> GPLSLSVDAFKILEDPKWEFPRKNLVLGKTLGEGEFGKVVKATAFHLKGRAGYTTVAVKMLKENASPSELRDLLSEFNVLKQVNHPHVIKLYGACSQDGPLLLIVEYAKYGSLRGFLRESRKVGPGYPDERALTMGDLISFAWQISQGMQYLAEMKLVHRDLAARNILVAEGRKMKISDFGLSRDVYEEDSYVKRSQGRIPVKWMAIESLFDHIYTTQSDVWSFGVLLWEIVTLGGNPYPGIPPERLFNLLKTGHRMERPDNCSEEMYRLMLQCWKQEPDKRPVFADISKDLEKMMVKR

RET (REarranged during Transfection) is a receptor tyrosine kinase (RTK) that is required for normal development, maturation and maintenance of several tissues and cell types. Gain of function mutations in RET are implicated in several human cancers, e.g. medullary thyroid cancer (MTC) and lung adenocarcinoma (LAD). The identification of these mutations and rearrangements in RET which lead to constitutive activation, together with convincing preclinical data validating RET as a classical oncogene, make this kinase an attractive target for cancer therapy. Our initial focus was to identify novel, low molecular weight, ATP-competitive inhibitors of the RET kinase domain with improved selectivity for RET against KDR in cellular assays, relative to 1.

Of the first swathe of approximately 30 simple anilinoquinazolines prepared, the most interesting observation was that phenol 6 resulted in a significant gain in affinity towards RET. The boost in RET affinity from the R2 hydroxyl group may be rationalised by consideration of the hydrogen bonding contacts formed in the gatekeeper pocket. Initial modelling of 6, subsequently confirmed by the determination of the X-ray structure bound to RET, highlighted a pair of hydrogen bonds from the phenol to the side-chain of Glu775 (the conserved glutamate located on the αC-helix) and the backbone NH of Asp892 (from the conserved DFG motif). Comparison of the X-ray structures of 6 and 1 reveals that the ligands share very similar binding modes. The quinazoline core binds to the hinge region (Glu805-Ala807), with the anilino ring enclosed within the hydrophobic pocket between the gatekeeper residue Val804 and the catalytic lysine Lys758. The anilino ring of 6 binds between the gatekeeper Val804 and the catalytic lysine Lys758 and, in comparison to 1, shows a small rotation towards Asp892, with minor re-orientation of neighbouring side-chains consistent with the formation of hydrogen-bonding interactions between the phenol and Glu775/Asp892. The most substantial structural change is the displacement of the phosphate-binding loop away from the ATP binding site in the X-ray structure of 6; this may be a consequence of a degree of induced fit in the ligand binding site or may simply reflect the inherent flexibility of this loop. Modelling of 6 in various published X-ray structures of KDR suggested that the hydrogen bonding network around the phenol in RET may be less readily achievable in KDR. This is a consequence of KDR X-ray structures displaying a conformation in which the αC-helix is displaced away from the ATP binding site in comparison to RET. The associated movement of the conserved glutamate located on the αC-helix (equivalent to Glu775 in RET) would likely compromise the formation of the pair of hydrogen bonds to the phenol observed crystallographically in RET.> MPELPEVEAARRAIEENCLGKKIKRVIIADDNKVIHGISPSDFQTSILGKTIISARRKGKNLWLELDSPPFPSFQFGMAGAIYIKGVAVTKYKRSAVKDSEEWPSKYSKFFVELDDGLELSFTDKRRFAKVRLLANPTSVSPISELGPDALLEPMTVDEFAESLAKKKITIKPLLLDQGYISGIGNWIADEVLYQARIHPLQTASSLSKEQCEALHTSIKEVIEKAVEVDADSSQFPSNWIFHNREKKPGKAFVDGKKIDFITAGGR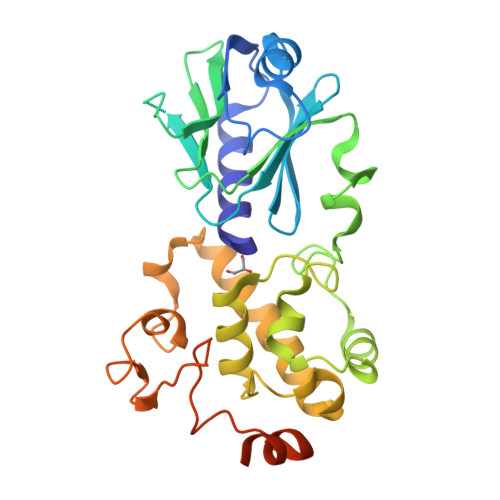TTAYVPELQKLYGKDAEKAAKVRPAKRGVKPKEDDGDHHHHHH> SLENENQLTHQFPTLSRWNPMFISDVHKISFHPHLQRYIGFWMGFPIRWIQIVGYIAAIDIYEGKHVLTVDDCSGMVLRVVFIIQDDFSMSKRA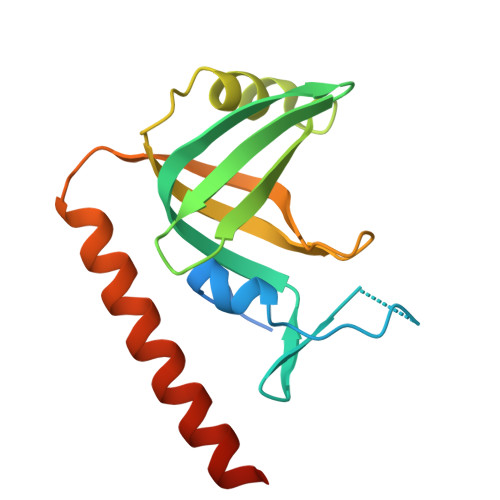ISMSPGNVVCVFGKINSFRSEVELIAQSFEELRDPNDEWKAWQKRMRYKKNLTKISKNHHSIIRT>STQQHTEPAEEETLHNIITDTENVQG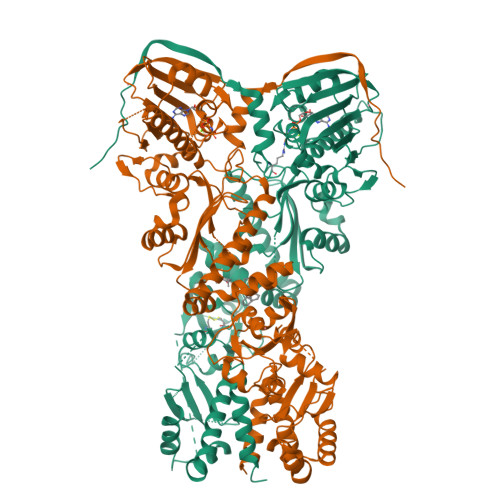SFSKHEFQAETKKLLDIVARSLYSEKEVFIRELISNGSDALEKLRHRMITAGGDTAPMEIHLQTDSVKGTFTIQDTGVGMNKEDLVSNLGTIARSGSKAFLDALQNQAEASSSIIGQFGVGFYSAFMVADKVEVYSQSAEADAPGYKWSSDGSGVFEVAEASGVRQGTKIVLHLKDDCKEFSSEDRVKEVVTKYSNFVSFPIFLNGRRLNTLQALWMMEPKDISEWQHEEFYRYVAQAYDKPRYTLHYRADAPLNIRSIFYVPEMKPSMFDVSREMGSSVALYSRKILIQTKATDILPKWLRFLRGVVDSEDIPLNLSRELLQESALIRKLRDVLQQRVIRFLLDQSKKDPEKYARFFEDYGLFMREGIVTTGEQSVKEDIAKLLRFESSALPAGQQTSLMEYSSRMKAGTRNIYYLCAPNRHLAEHSPYFEAMKQKDMEVLFCFEQFDELTLLHLREFDRKKLISAETDIVVDHYKEEKFQDSKPASERLSSEQAEDLLAWMRNALVQRVTNIKVTPRLDTHPAMITVLEMGAARHFLRTQQLARSSEERAQILQPTLEINTGHDLIKKLHALKDSNPELAQLLLEQIYDNAMIAAGLNEDPRPMISRLNQLLTRALEKH[2x]>ATANLHLYQDLQREVGSLKEINFMLSVLQKEFLHLSKEFATTSKDLSAVSQDFYSCLQAFRDNYKGFESLLDEYKNSTEEMRKLFSQEIIADLKGSVASLREEIRFLTPLAEEVRRLAHNQQSLTAAIEELKTIRDSLRDEIGQLSQLSKTLTSQIALQRKLEHHHHHH[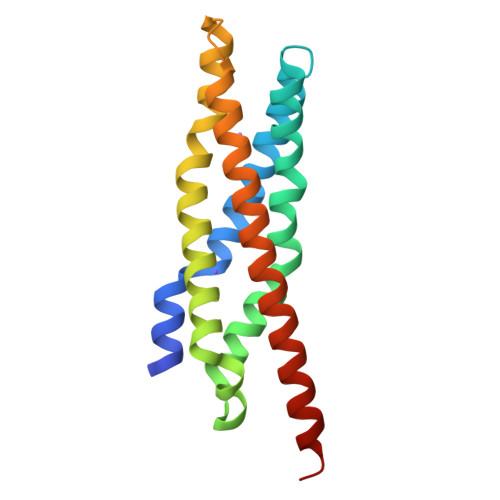2x]>MLENYARFITAASAARNPSPIRTMTDILSRGPKSMISLAGGLPNPNMFPFKTAVITVENGKTIQFGEEMMKRALQYSPSAGIPELLSWLKQLQIKLHNPPTIHYPPSQGQMDLCVTSGSQQGLCKVFEMIINPGDNVLLDEPAYSGTLQSLHPLGCNIINVASDESGIVPDSLRDILSRWKPEDAKNPQKNTPKFLYTVPNGNNPTGNSLTSERKKEIYELARKYDFLIIEDDPYYFLQFNKFRVPTFLSMDVDGRVIRADSFSKIISSGLRIGFLTGPKPLI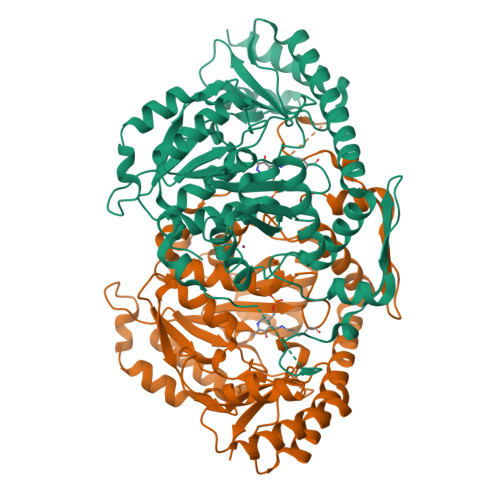ERVILHIQVSTLHPSTFNQLMISQLLHEWGEEGFMAHVDRVIDFYSNQKDAILAAADKWLTGLAEWHVPAAGMFLWIKVKGINDVKELIEEKAVKMGVLMLPGNAFYVDSSAPSPYLRASFSSASPEQMDVAFQVLAQLIKESL[2x]> GSHMEAVQNRIVEAAERVPGVRGVIHLRARYVGQDIWADMIIGVDPENTVEQAHEICEAVQAAVCGKIRRIESLHVSAAAREIGDTTKPSFSDQPLSFDEVMLSKVDN

One group of metal ion efflux transporters that regulates metal ion homeostasis and can be found in all domains of life is the Cation Diffusion Facilitator (CDF) protein family. One of the most highly conserved and abundant integral MM proteins is the CDF transporter MamM. MamM was recently proposed to function as a magnetosome-directed iron transporter required for iron biomineralization since its deletion abolished magnetite biomineralization and mutation of residues within the conserved TMD metal-binding site resulted in alterations of magnetite crystal size, morphology and even mineral phase. To summarize our results we present an alternative model for the CDF CTD mode of action, in which we propose that upon metal cation binding, the CTD induces conformational changes towards a tighter and more compact fold which allows the activation of iron transport through the TMD.

Examining this closed state model, three putative binding sites were revealed, in which Asp, Glu and His residues from the two monomers are brought into close proximity and may bind divalent cations. The other two symmetrical peripheral binding sites contain His264 and Glu289 residues but no designated binding cavity was found. In contrast, E289A from the peripheral binding sites resulted in a significantly lower magnetic response that correlated with a significantly lower number of magnetite particles per cell (−17%; P<0.01, Mann-Whitney test). However, size and shape of the particles were unaffected in E289A mutants. Furthermore, only the D249A and E289A single mutants revealed an additional slight decrease of the magnetic response during iron induction experiments with iron-starved cells. Whereas, only in the E289A mutant was the number of binding sites significantly reduced (2.0±0.2). Since Glu289 is located at the domain surface, it is more likely to have a role in peripheral binding site stabilization and metal ion coordination than the relatively buried His264. To confirm that these observed phenotypic differences are due to true transport function alternations, we also examined the expression levels of all MamM mutants, their ability to stabilize MamB expression, performed MD simulations for dimer stability evaluation and determined their CTD structures. (ii) All mutants exhibited an apo-MamM CTD-like behavior along the MD simulations (see Fig. B in file S1 for representative MD simulations), and (iii) an absence of structural differences was observed.> EVHSRGQFIEQPNSVECDF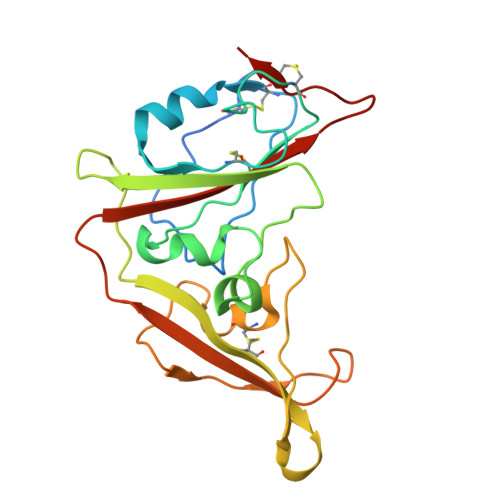TKLLSGTPPQVYNFNRLVFTNCNYNLTKLLSLFMVNEFSCDGISPDAIARGCYSSLTVDYFAYPLSMKSYMQPGSAGVISQYNYKQSFANPTCRIFATAPANLTITKPSSYSFISKCSRLTGDNSHIETPIVINPGEYSICKNFAPNGFSQDGDYFTRQLSQLEGGGILVGVGSVTPMTDTLQMGFIISVQYGTDTNSVCPMMD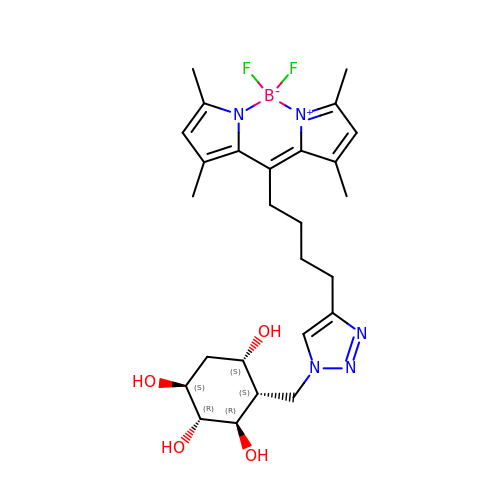(1~{S},2~{R},3~{R},4~{S},5~{S})-4-[[4-[4-[2,2-bis(fluoranyl)-4,6,10,12-tetramethyl-3-aza-1-azonia-2-boranuidatricyclo[7.3.0.0^{3,7}]dodeca-1(12),4,6,8,10-pentaen-8-yl]butyl]-1,2,3-triazol-1-yl]methyl]cyclohexane-1,2,3,5-tetrol | C26 H36 B F2 N5 O4 | FESFUVRFRDTLFV-GZBLQCQNSA-N1-{4-[6-amino-5-(4-chlorophenyl)pyridin-3-yl]phenyl}cyclopentane-1-carboxylic 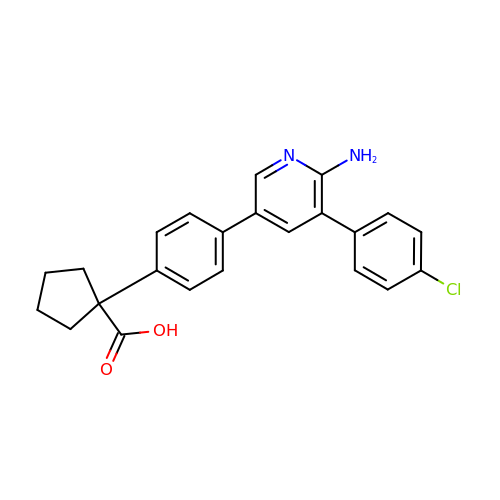acid | C23 H21 Cl N2 O2 | VHQILBJBMFWZGW-UHFFFAOYSA-N>[3x]GSHMASNKYKRIFLVVMDSVGIGEAPDAEQFGDLGSDTIGHIAEHMNGLQMPNMVKLGLGNIREMKGISKVEKPLGYYTKMQEKSTGKDTMTGHWEIMGLYIDTPFQVFPEGFPKELLDELEEKTGRKIIGNKPASGTEILDELGQEQMETGSLIVYTSADSVLQIAAHEEVVPLDELYKICKIARELTLDEKYMVGRVIARPF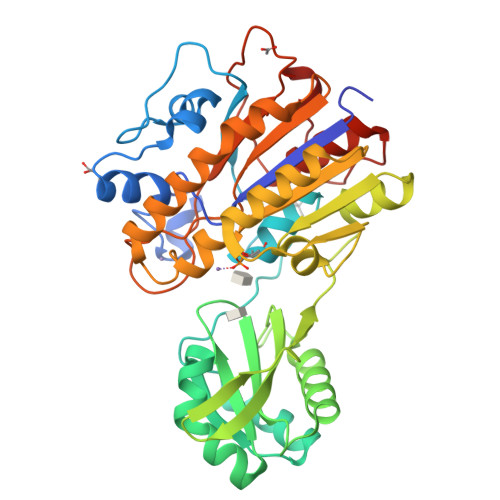VGEPGNFTRTPNRHDYALKPFGRTVMNELKDSDYDVIAIGKISDIYDGEGVTESLRTKSNMDGMDKLVDTLNMDFTGLSFLNLVDFDALFGHRRDPQGYGEALQEYDARLPEVFAKLKEDDLLLITADHGNDPIHPGTDHTREYVPLLAYSPSMKEGGQELPLRQTFADIGATVAENFGVKMPEYGTSFLNELKK>MSNHTYRVTDIVGTSP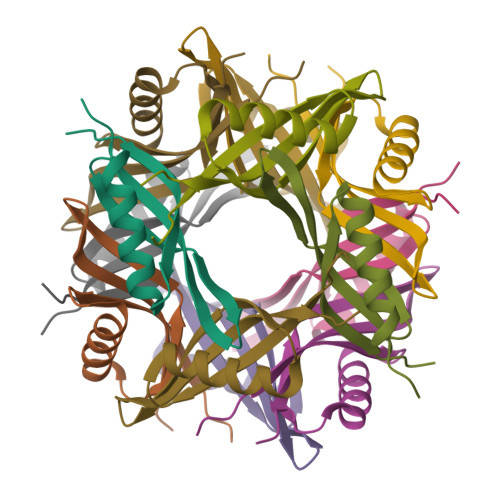EGVDQAIRNGINRASQTLHNLDWFEVVEVRGQLNDGQIAHWQVTMKVGFRLDETG[6x]>PCLTGPRTCKDLLDRGHFLSGWHTIYLPDCRPLTVLCDMDTDGGGWTVFQRRVDGSVDFYRDWATYKQGFGSRLGEFWLGNDNIHALTAQGTSELRVDLVDFEDNYQFAKYRSFKVADEAEKYNLVLGAFVEGSAGDSLTFHNNQSFSTKDQDNDLNTGNCAVMFQGAWWYKNCHVSN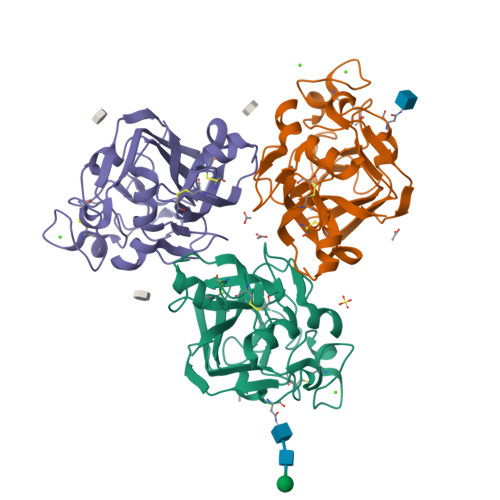LNGRYLRGTHGSFANGINWKSGKGYNYSYKVSEMKVRPA[3x]> MAHHHHHHAQPVLDAPAPGPDTPEAASGPGLLFADEFDGPAGSPPDPAKWFIVPERETIRNPVEWDKPYNMGRYVTDQEHVFHDGNGNLVIRATRGPGANIREKYASAKIVGLWRGGVGTTWEARVKLNCLTDGAWPAFWLLNDDPVRGAEIDIFEWYGNRDWPSGATVHAKLDGTMF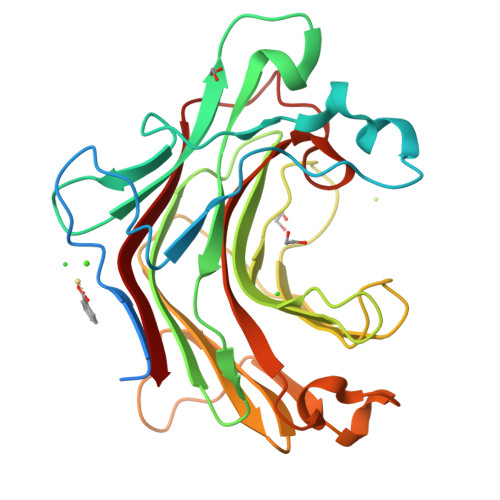QTQNYPVDSAWHTWRMTWLPSGMYFWQDYEPGKEPFFTVLANSLPEWPFNDPGYTMVPVFNIAVGGSGGREPAGGSYPADMIIDWIRVF> MNNNKAEADTSSSMADPETRPTYTTHHLAIPSGVTQDEFDELKQSVVEFHTYQLSQAQCSSLLAQRIRAPNDVVWSIVRRFDQPQTYKHFIKSCSVSDNFTMAVGSTRDVNVISGLPAATSTERLDILDDDRQVTGFSIIGGEHRLRNYRSVTSVHGFNRDGAICTVVLESYVVDVPEGNTEEDT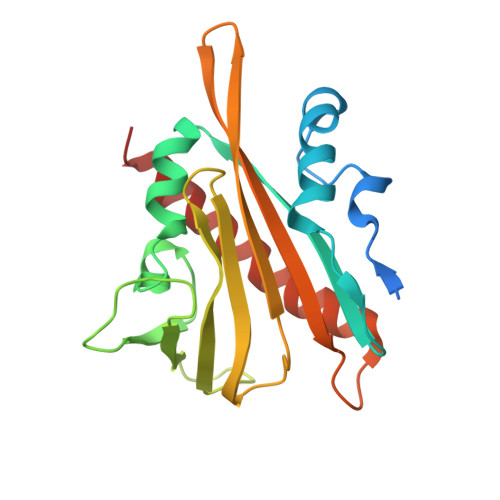RLFADTVVKLNLQKLVSVAESQVI>MGSSHHHHHHSQDPMSTGTFVVSQPLNYRGGARVEPADASGTEKAFEPATGRVIATFTCSGEKEVNLAVQNAKAAFKIWSQKSGMERCRILLEAARIIREREDEIATMECINNGKSIFEARLDIDISWQCLEYYAGLAASMAGEHIQLPGGSFGYTRREPLGVCVGIGAWNYPFQIASWKSAPALACGNAMVFKPSPFTPVSALLLAEIYSEAGVPPGLFNVVQGGAATGQFLCQHPDVAKVSFTGSVPTGMKIMEMSAKGIKPVTLELGGKSPLIIFSDCDMNNAVKGALMANFLTQGQVCCNGTRVFVQKEILDKFTEEVVKQTQRIKIGDPLLEDTRMGPLINRPHLERVLGFVKVAKEQGAKVLCGGDIYVPEDPKLKDGYYMRPCVLTNCRDDMTCVKEEIFGPVMSILSFDTEAEVLERANDTTFGLAAGVFTRDIQRAHRVVAELQAGTCFINNYNVSPVELPFGGYKKSGFGRENGRVTIEYYSQLKTVCVEMGDVESAF[8x]

Aldehyde dehydrogenases (ALDHs) catalyze the NAD(P)+-dependent irreversible oxidation of aliphatic and aromatic aldehydes. Human ALDH9A1 is a cytosolic tetrameric enzyme of ∼216 kDa that was first purified from the liver and characterized as a 4-aminobutyraldehyde (ABAL) dehydrogenase (ABALDH, E.C. 1.2.1.19). The enzyme is involved in the carnitine synthesis pathway comprising three other enzymes: trimethyl lysine dioxygenase, 3-hydroxy-N-trimethyllysine aldolase and γ-butyrobetaine (TMABA) dioxygenase. In the present study, using kinetic assays and affinity measurements, we showed that among various available aminoaldehydes, ALDH9A1 preferentially oxidizes TMABAL with the highest rates at very low saturating micromolar concentrations.

Co-crystallization with 50 mM NAD+ with or without 10 mM TMABA product resulted into different crystal forms. However, the three solved structures from P21212, P21, and C2 space groups at 2.5, 2.9, and 2.3 Å, respectively, reveal an ALDH9A1 apoform in the absence of a bound NAD+ or TMABA. The asymmetric units of the P21212 and P21 structures contain two similar tetramers (dimer-of-dimers) and that of C2 only one. All monomers are very similar to each other with an RMSD up to 0.24 Å. Each monomer displays the classical ALDH fold consisting of a catalytic domain (residues 258–448) with the catalytic Cys288, a coenzyme binding domain (residues 1–127, 146–257, 470–478), and an oligomerization domain (residues 128–145 and 479–494), which wraps over the groove between the catalytic and coenzyme domains of the other monomer forming the dimer. The αβE region is not visible in the electron density maps thus is highly mobile. The first one concerns the αβE region, which is composed of the α-helix E and β-strand E, located at the dimer interface. This region interacts with the bound NAD+ when present in ALDH structures, and the absence of a bound NAD+ in the HsALDH9A1 structure is in agreement with this largely disordered region. In our three HsALDH9A1 structures, the inter-domain linker adopts a unique fold, never observed so far, preventing the binding of any substrate. The same fold of the inter-domain linker in the three crystal forms suggests that this linker exhibits such conformation in the apoform. Therefore, a switch corresponding to a rearrangement up to 30 Å must occur for substrate binding followed by NAD+ binding.IRE1α, the most evolutionarily conserved UPR sensor that is ubiquitously expressed, consists of the N-terminal ER luminal domain that senses unfolded proteins and the C-terminal cytoplasmic region that includes the serine/threonine kinase domain and the endoribonuclease (RNase) domain, exhibiting dual kinase and endoribonuclease functions. IRE1α oligomerization and autophosphorylation under ER stress activate its endoribonuclease activity via binding and cleaving RNA substrates, triggering downstream UPR pathways. For example, IRE1α induces splicing of the X-box-binding protein 1 (XBP1) mRNA that encodes the transcription factor XBP1 spliced isoform protein (XBP1), which upregulates genes involved in the ER protein folding and secretion, promotes degradation of misfolded proteins, and further relieves ER stress.

The obtained structure contained four copies within the asymmetric unit, chain A and chain B formed a back-to-back dimer, and chain C formed the same dimer with chain D from the molecule in the next asymmetric unit. The propionic acid group of IA107 extends towards the pocket proximal to the DFG-motif (Asp-Phe-Gly, residue 711-713), which is a conserved motif located at the beginning region of the kinase activation loop. The N-benzoyl motif of IA107 faces towards the adenine pocket and interacts with the kinase hinge region. Crucial hydrogen bond interactions were formed between the propionic acid of IA107 with the backbone of D711 and with the catalytic K599. Another important hydrogen bond was formed between the carbonyl amide of IA107 and the backbone of C645. IA107 interacts with K599 with the observed N-terminal αC-helix shift upon IA107 binding, and the salt bridge between K599 and E612 of the αC-helix remains intact. The conserved DFG motif does not show any significant shift when aligned with the IA107-binding p-IRE1α structure with the apo form structure, with the DFG-motif adopting a DFG-in conformation in both structures. Despite that the interaction of the two protomers of the kinase domain remains the same, the IA107-binding leads to a more separated conformation between the two RNase domains (835-963) with a reduced overall interaction interface. The kinase domains of the two protomers interact with each other in the back-to-back dimeric conformation upon IA107 binding, maintaining the dimeric and oligomeric assemblies of p-IRE1α but the RNase domains are more separated, resulting in the inhibition of the RNase activity of IRE1α. The binding of IA107 did not impact the formation of the Lys–Glu bridge and the high-order assembly of IRE1α, instead, IA107 inhibited the RNase activity by separating the RNase domain dimer interface, confirming the formation of the RNase dimer is critical for the IRE1 RNase activity.

>[4x]GGSGSSPSLEQDDGDEETSVVIVGKISFCPKDVLGHGAEGTIVYRGMFDNRDVAVKRILPECFSFADREVQLLRESDEHPNVIRYFCTEKDRQFQYIAIELCAATLQEYVEQKDFAHLGLEPITLLQQTTSGLAHLHSLNIVHRDLKPHNILISMPNAHGKIKAMISDFGLCKKLAVGRHSFSRRSGVPGTEGWIAPEMLSEDCKENPTYTVDIFSAGCVFYYVISEGSHPFGKSLQRQANILLGACSLDCLHPEKHEDVIARELIEKMIAMDPQKRPSAKHVLKHPFFWSLEKQLQFFQDVSDRIEKESLDGPIVKQLERGGRAVVKMDWRENITVPLQTDLRKFRTYKGGSVRDLLRAMRNKKHHYRELPAEVRETLGSLPDDFVCYFTSRFPHLLAHTYRAMELCSHERLFQPYYFHEPPEPQPPVTPDAL> MPQLEASLELDFQSESYKDAYSRINAIVIEGEQEAFDNYNRLAEML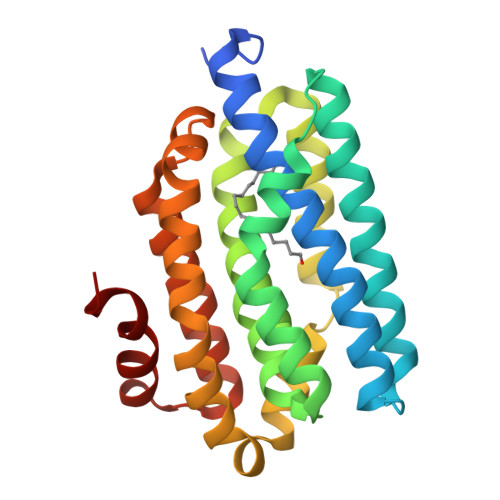PDQRDELHKLAKMEQRHMKGFMACGKNLSVTPDMGFAQKFFERLHENFKAAAAEGKVVTCLLIQSLIIECFAIAAYNIYIPVADAFARKITEGVVRDEYLHRNFGEEWLKANFDASKAELEEANRQNLPLVWLMLNEVADDARELGMERESLVEDFMIAYGEALENIGFTTREIMRMSAYGLAAV> GMQQVIKDLFYVVPLSRNCEKIYKNKTHILLGISPFNSKFSQNYIHQLIDWSSKNFKNVTVLLAGDEAKNLLEALGTPTTKAERKVRKEIRRHFRFSEEALRKNGREIDIYTFSDFKNNKIYNEVYQNVIYYFEKDEKFRKSCLAMSHDALSSRAKSLNMEDIEITDNMLFHAVKYVLAELPFFLSGASILGYKESVLAYHRPWKLGE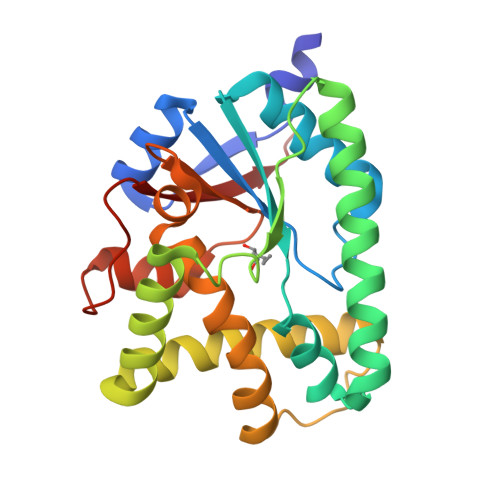KIKNSEFYIKMSDNQGYIILKQIN>[2x]MGLAVFLPPYPFRGLKAPYLWMFYKYLHCATDSILFITGEDYLSVTDDEAQRARWEFDPASMASLGYELPNAQSMACHEYLTLDNAFYETLLSRHHHDPIKSFSAFLTERIPDLETELHALLDSKKGIIDQIDT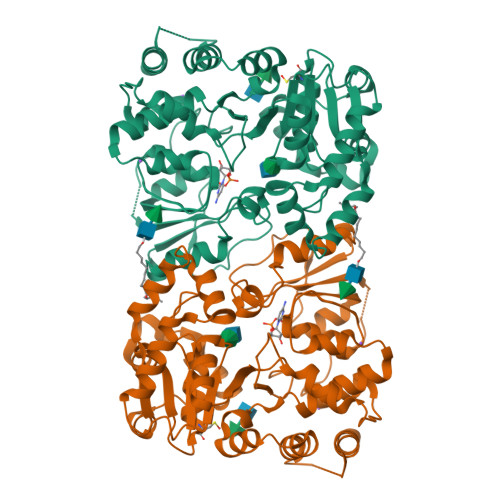FISICNCPSLEHVARTLGKEVMHIEIGPLRAPMYRNTAYLDFAGVNGGTEASARYEKCQAEFDIKASLGDLHNYFLEVLPPAEAATHSAAGVVLQVEDDSNLIAYNHDFTNISLLSYVRQRYEKEDILVRAHPGSLFRLRDDVFTIDDSANSLAFINQCNEVFTINSSVGLEAILTGKKTTVLGDCSYAFINELAGASATVNAAAFYLFSYLVPFDLVFNQEYLKFRLGHPEEREIVGKHIEFYSADMPGSLSQAASSLSSLINEAISLEHHHHHH> MSNISRQAYADMFGPTVGDKVRLADTELWIEVEDDLTTYGEEVKFGGGKVIRDGMGQGQMLAADCVDLVLTNALIVDHWGIVKADIGVKDGRIFAIGKAGNPDIQPNVTIPIGAATEVIAAEG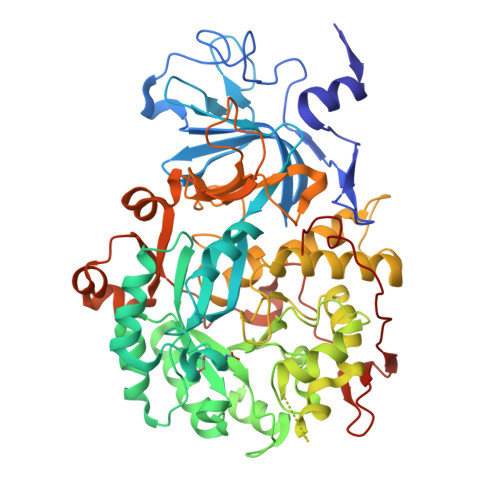KIVTAGGIDTHIHWICPQQAEEALVSGVTTMVGGGTGPAAGTHATTCTPGPWYISRMLQAADSLPVNIGLLGKGNVSQPDALREQVAAGVIGLKIHEDWGATPAAIDCALTVADEMDIQVALHSDTLNESGFVEDTLAAIGGRTIHTFHTEGAGGGHAPDIITACAHPNILPSSTNPTLPYTLNTIDEHLDMLMVCNHLDPDIAEDVAFAESRIRRETIAAEDVLHDLGAFSLTSSDSQAMGRVGEVILRTWQVAHRMKVQRGALAEETGDNDNFRVKRYIAKYTINPALTHGIAHEVGSIEVGKLADLVVWSPAFFGVKPATVIKGGMIAIAPMGDINASIPTPQPVHYRPMFGALGSARHHCRLTFLSQAAAANGVAERLNLRSAIAVVKGCRTVQKADMVHNSLQPNITVDAQTYEVRVDGELITSEPADVLPMAQRYFLF> MAGAIASRMSFSSLKRKQPKTFTVRIVTMDAEMEFNCEMKWKGKDLFDLVCRTLGLRETWFFGLQYTIKDTVAWLKMDKKVLDHDVSKEEPVTFHFLAKFYPENAEEELVQEITQHLFFLQVKKQILDEKIYCPPEASVLLASYAVQAKYGDYDPSVHKRGFLAQEELLPKRVINLYQMTPEMWEERITAWYAEHRGRARDEAEMEYLKIAQDLEMYGVNYFAIRNKKGTELLLGVDALGLHIYDPENRLTPKISFP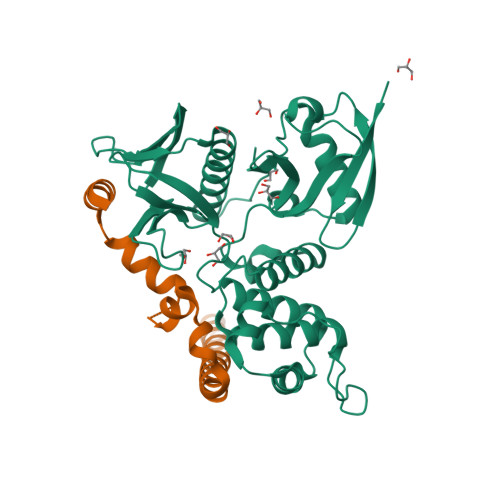WNEIRNISYSDKEFTIKPLDKKIDVFKFNSSKLRVNKLILQLCIGNHDLFMRRRKADSLEVQQ;> SFDFKDTDMKRLDMEIEKEKVEYMEKSKHLQEQLNELKTEIEALKLKERETALDILHNENSDRGGSSKHNTIKKLTLQSWKSRVAFFEEL>[2x]GPGSMRFENKVGIVTGSGGGIGQAYAEALAREGAAVVVADINAEAAEAVAKQIVADGGTAISVAVDVSDPESAKAMADRTLAEFGGIDYLVNNAAIFGGMKLDFLLTIDPEYYKKFMSVNLDGALWCTRAVYKKMTKRGGGAIVNQSSTAAWLYSNYYGLAKVGINGLTQQLSRELGGRNIRINAIAPGPIDTEANRTT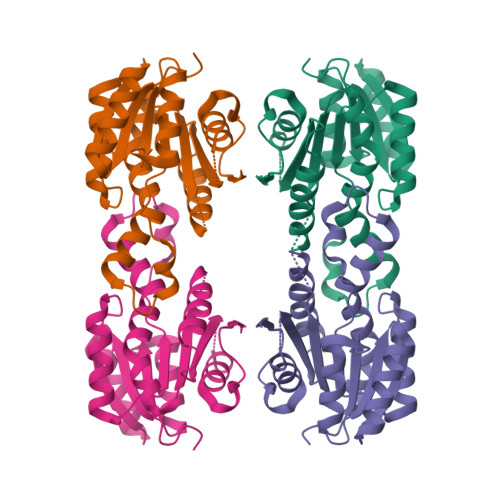TPKEMVDDIVKGLPLSRMGTPDDLVGMCLFLLSDEASWITGQIFNVDGGQIIRS> QVRPFLDVYQRSACQTRETLVSILQEHPDEISDIFRPSCVAVLRCSGCCTDESMKCTPVGKHTADIQIMR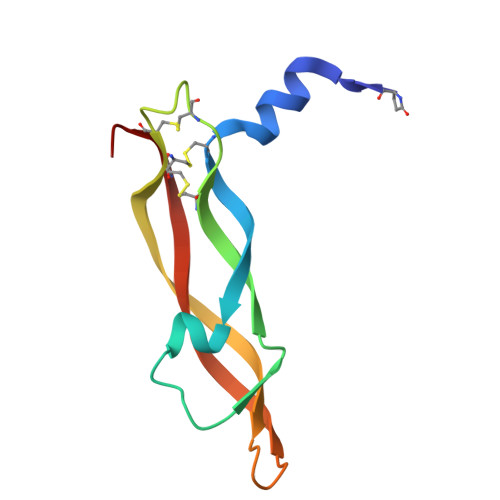MNPRTHSSKMEVMKFMEHTACECRPA>[6x]MTQFNITWEEQLQALSKLDGLHHPHKLEDISVHWVFNPVDISVFVTCATMSSHNTHYTFKPQSSPDDA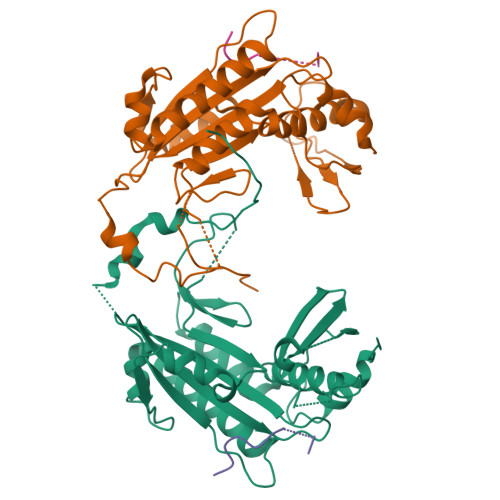MVREYVLSRIIADNLKYVDNLYLAAGAVICGNDEYISDGNVVGIHIADGVGGNKLILPVIEFMPGVHVDDISDKLIKSSSYQGIFKTDNLEEFEFLVDKKNANNVKELILAYTDYFANKLAFKDPAEPAVEMYQFIDRTEVYFSFEGCHPDVEEVLFTIKIVRYNQPLNSTAMQVFLKNPLLSHIRTVVRQDLPAKFVGGVLFNFKGHHHHHH;>[6x]ERPRRRSRGQRRRSNRRERQ>[3x]MFEARLVQGSILKKVLEALKDLINEACWDISSSGVNLQSMDSSHVSLVQLT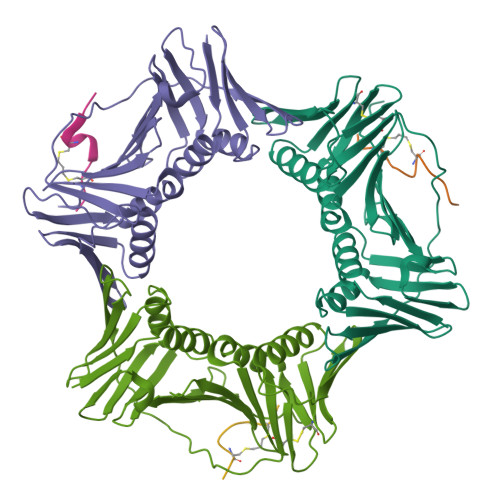LRSEGFDTYRCDRNLAMGVNLTSMSKILKCAGNEDIITLRAEDNADTLALVFEAPNQEKVSDYEMKLMDLDVEQLGIPEQEYSCVVKMPSGEFARICRDLSHIGDAVVISCAKDGVKFSASGELGNGNIKLSQTSNVDKEEEAVTIEMNEPVQLTFALRYLNFFTKATPLSSTVTLSMSADVPLVVEYKIADMGHLKYYLAPKIEDE;>[3x]XRQCSMTCFYHSKX> EEATSKGQNLNVEKINGEWFSILLASDKREKIEEHGSMRVFVEHIHVLENSLAFKFHTVIDGECSEIFLVADKTEKAGEYSVMYDGFNTFTILKTDYDNYIMFHLINEKDGKTFQLMELYGRKADLNSDIKEKFVKLCEEHGI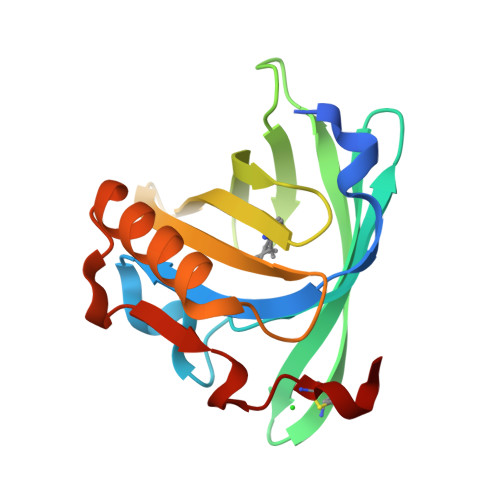IKENIIDLTKTNRCLKARE GAMMA-GLUTAMYL PHOSPHATE | C5 H10 N O7 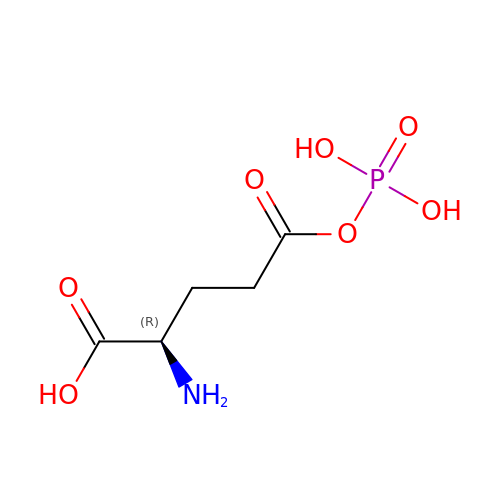P | PJRXVIJAERNUIP-GSVOUGTGSA-N> AGTHDYSTALKDSIIFFDANKCGPQAGENNVFDWRGACHTTDGSDVGVDLTGGYHDAGDHVKFGLPQGYSAAILGWSLYEFKESFDATGNT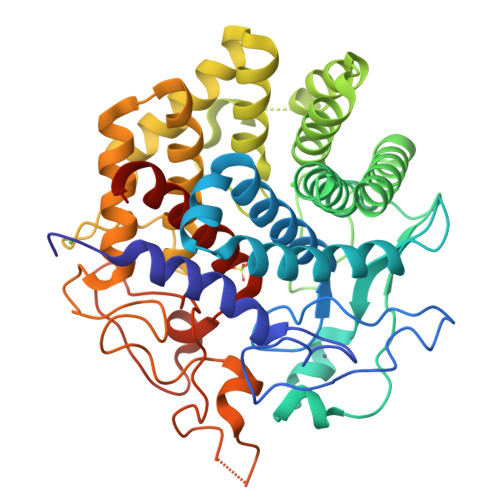TKMLQQLKYFTDYFLKSHPNSTTFYYQVGEGNADHTYWGAPEEQTGQRPSLYKADPSSPASDILSETSAALTLMYLNYKNIDSAYATKCLNAAKELYAMGKANQGVGNGQSFYQATSFGDDLAWAATWLYTATNDSTYITDAEQFITLGNTMNENKMQDKWTMCWDDMYVPAALRLAQITGKQIYKDAIEFNFNYWKTQVTTTPGGLKWLSNWGVLRYAAAESMVMLVYCKQNPDQSLLDLAKKQVDYILGDNPANMSYIIGYGSNWCIHPHHRAANGYTYANGDNAKPAKHLLTGALVGGPDQNDKFLDDANQYQYTEVALDYNAGLVGVLAGAIKFFGGTIVNPPVKK>[6x]GSHMRAEERERLAEVEAALEKQRQLA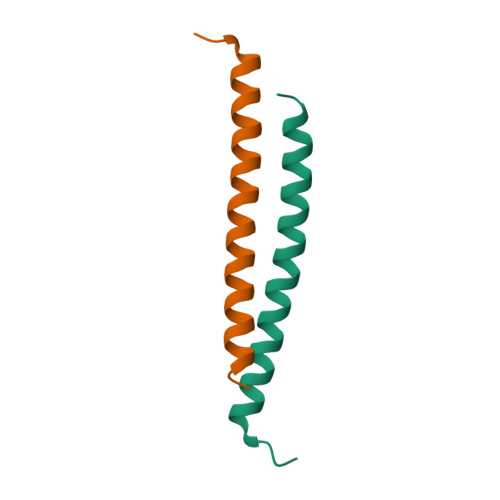EAHAQAKAQAEREAKEL> GSHMKNSVSVDLPGSMKVLVSKSSNADGKYDLIATVDALELSGTSDKNNGSGVLEGVKADASKVKLTISDDLGQTTLEVFKSDGSTLVSKKVTSKDKIIIIIKFNEKGEVSEKIITRADGTRLEYTG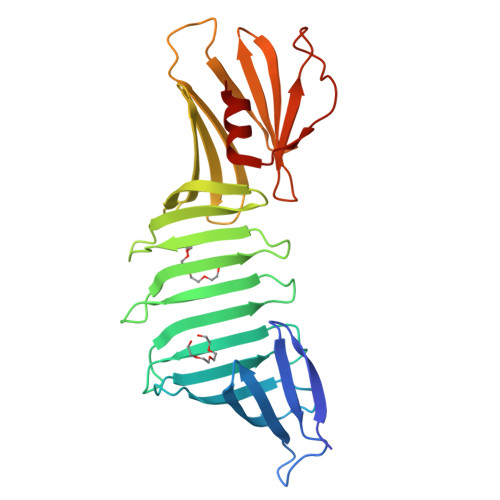IKSDGSGKAKEVLKGYVLEGTLTAEKTTLVVKEGTVTLSKNISKSGEVSVELNDTDSSAATKKTAAWNSGTSTLTITVNSKKTKDLVFTSSNTITVQQYDSNGTSLEGSAVEITKLDEIKNALK> 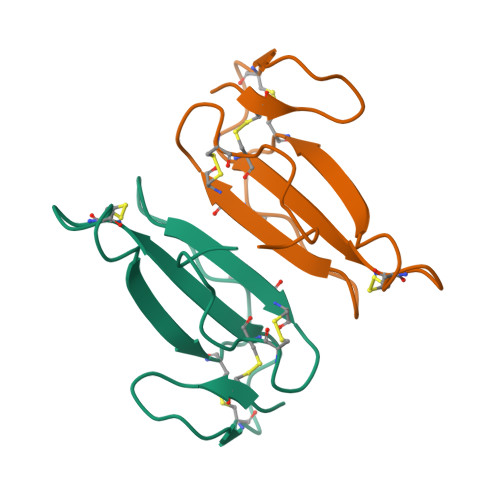IRCFITPDITSKDCPNGHVCYTKTWCDAFCSIRGKRVDLGCAATCPTVKTGVDIQCCSTDNCNPFPTRKRP> TNMGLEAIIRKALM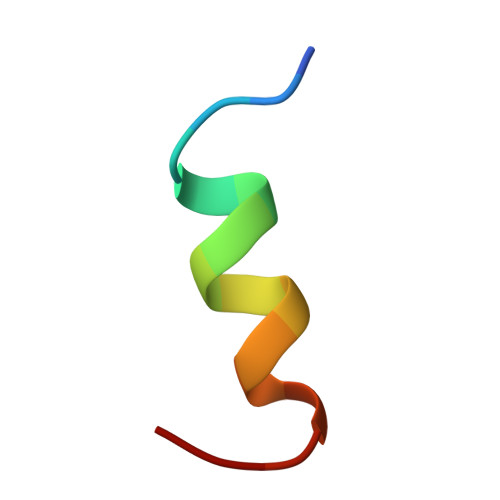GK> KLTKEELKEIVTMMVNKLTNRLSEQNINIIVTDKAKDKIAEEGYDPEYGARPLIRAIQKTI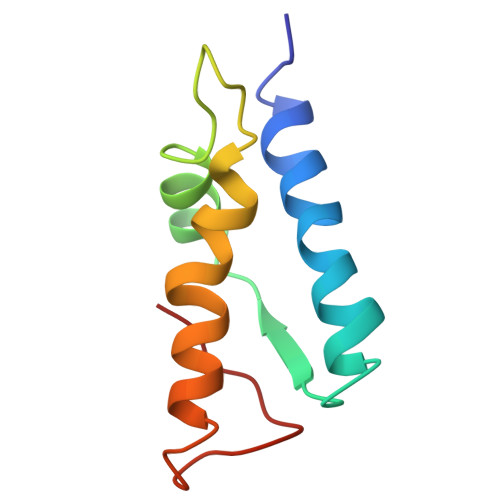EDNLSELILDGNQIEGKKVTV[(1R,2S,4S)-2-bicyclo[2.2.1]heptanyl] 4-azanylbenzoate | C14 H17 N O2 | 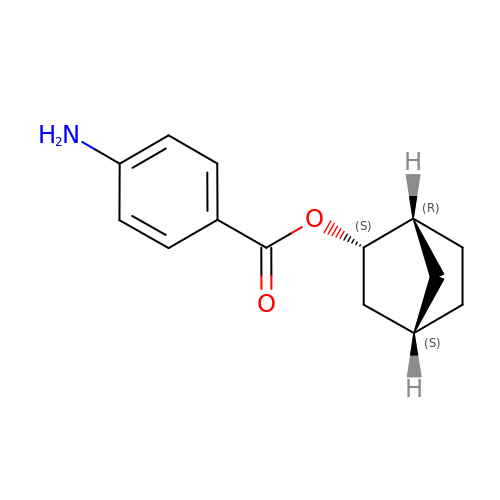GVFBCMCEUNYYSX-NDMJEZRESA-N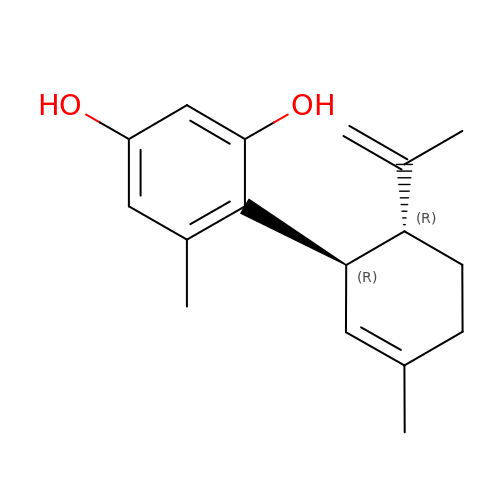(1'R,2'R)-5',6-dimethyl-2'-(prop-1-en-2-yl)-1',2',3',4'-tetrahydro[1,1'-biphenyl]-2,4-diol | C17 H22 O2 | KDZOUSULXZNDJH-LSDHHAIUSA-N> MGMRGSHHHHHHRPECVVPEFQCAVKRKEKKAQKDKDKPNSTTSCSPDGIKQEIDPQRLDTDSQLLSVNGVKPITPEQEELIHRLVYF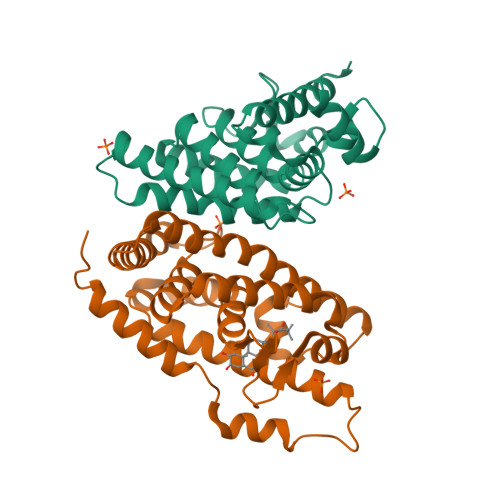QNEYEHPSPEDIKRIVNAAPEEENVAEERFRHITEITILTVQLIVEFSKRLPGFDKLIREDQIALLKACSSEVMMFRMARRYDAETDSILFATNQPYTRESYTVAGMGDTVEDLLRFCRHMCAMKVDNAEYALLTAIVIFSERPSLSEGWKVEKIQEIYIEALKAYVENRRKPYATTIFAKLLSVLTELRTLGNMNSETCFSLKLKNRKVPSFLEEIWDVVS;> MDYKDDDDKGPKREAVQEERQRNKEKSENEVESTSNSQNDMPIERILEAELRVEPKNEDIDSRDPVSDICQAADRQLYQLIEWAKHIPHFTELPVEDQVILLKSGWNELLIAGFSHRSMSVKDGIMLATGLVVHRNCAHQAGVGAIFDRVLTELVAKMREMKMDKTELGCLRSIVLFNPEAKGLKSTQQVENLREKVYAILEEYCRQTYPDQSGRFAKLLLRLPALRSIGLKCLEHLFFFKLVGNTSIDSFLLSMLESNSDS>[2x]MGDVKNFLYAWCGKRKMTPSYEIRAVGNKNRQKFMCEVQVEGYNYT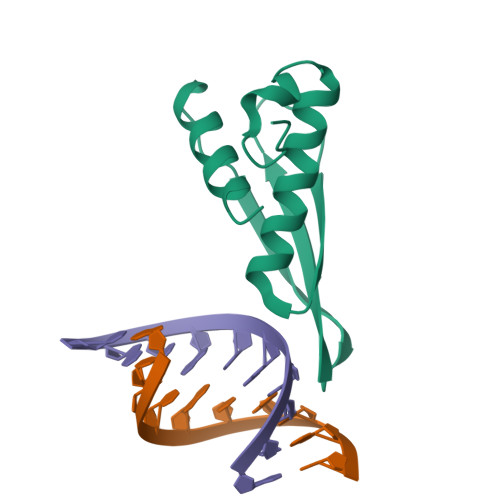GMGNSTNKKDAQSNAARDFVNYLVRINEIKSEEVPAFGVASPPPL>KKSIPVRGAAIFNENLSKILLVQGTESDSWSFPRGKISKDENDIDCCIREVKEQIGFDLTDY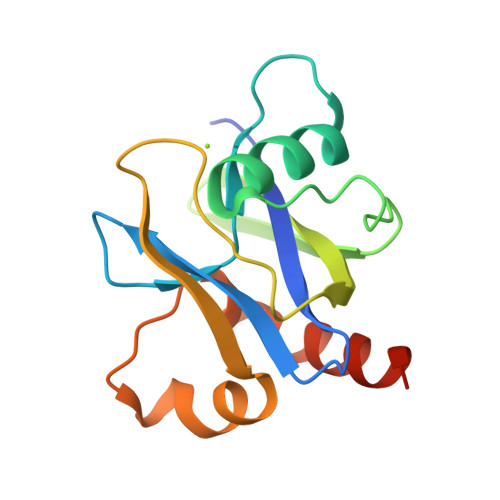IDDNQFIERNIQGKNYKIFLISGVSEVFNFKPQVRNEIDKIEWFDFKKISKTMYKSNIKYYLINSMMRPLSMWLRHQRQIKNED[3x]>GMSTFRQEDVEDHYEMGEELGSGQFAIVRKCRQKGTGKEYAAKFIKKRRLSSSRRGVSREEIEREVNILREIRHPNIITLHDIFENKTDVVLILELVSGGELFDFLAEKESLTEDEATQFLKQILDGVHYLHSKRIAHFDLKPENIMLLDKNVPNPRIKLIDFGIAHKIEAGNEFKN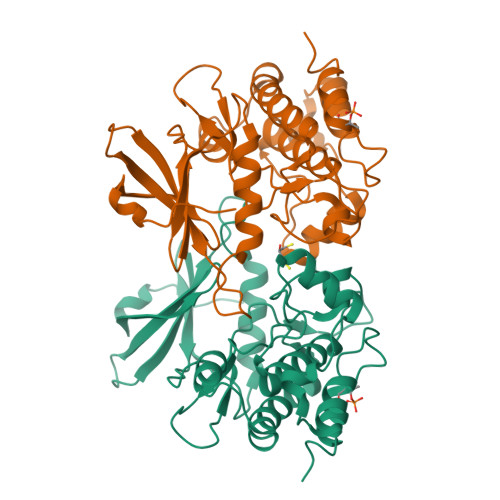IFGTPEFVAPEIVNYEPLGLEADMWSIGVITYILLSGASPFLGETKQETLTNISAVNYDFDEEYFSNTSELAKDFIRRLLVKDPKRRMTIAQSLEHSWIKA[2x]FtsEX is a membrane complex widely conserved across diverse bacterial genera and involved in critical processes such as recruitment of division proteins and in spatial and temporal regulation of muralytic activity during cell division or sporulation. The component FtsX is an integral membrane protein, whereas FtsE is an ATPase and is required for the transmission of a conformational signal from the cytosol through the membrane to regulate the activity of cell wall hydrolases in the periplasm. Here, we provide the first three-dimensional (3D) structure of FtsE from the notorious pathogen S. pneumoniae, and we show that it presents all the conserved structural motifs of the NBD members of the ABC transporter family. The nucleotide-binding site is located in lobe I near the interface between the two lobes and presents the nucleotide sandwiched between the Walker A and B motifs.

FtsE was crystallized with ADP in two different crystal forms (P 1 and P 21) and with AMP-PNP, a nonhydrolyzable analog of ATP, in the space group P 21. The FtsE–AMP-PNP complex was obtained by soaking with the P 21 FtsE-ADP crystals. The ATP analog was found in two out of the three independent monomers of the P 21 crystal. Structural comparison between our ADP and AMP-PNP complexes revealed that there were no relevant structural rearrangements directly associated with AMP-PNP binding, e.g., monomer M2 in complex with ADP and that in complex with AMP-PNP were nearly identical (RMSD of 0.22 Å for 223 Cα atoms). In the presence of AMP-PNP, K43 interacts with both the β- and γ-phosphates. The γ-phosphate is further stabilized by a direct interaction with the switch histidine (H197) and with S39. The catalytic glutamate (E165) is positioned directly adjacent to the γ-phosphate, consistent with a role in ATP hydrolysis. In conclusion, the residues that recognize the ATP molecule are properly oriented, and no relevant changes were required for nucleotide exchange. Other conclusions can be drawn from our structures; in particular, we have observed that while the relaxed structure of the FtsE-ADP complex nicely fits the equivalent complex in the MacB dimer; the monomer of the FtsE–AMP-PNP complex requires rigid-body adjustment of some regions around the central β-sheet in order to get a perfect fit with the more compact structure of the MacB-ATP dimer. For instance, in our FtsE–AMP-PNP complex, the γ-phosphate is far from the Q88 residue of the Q-loop (>6 Å); however, our composite model for the same structure in the dimer indicates that Q88 would directly recognize the γ-phosphate, as also occurs in the structure of the MacB-ATP dimer.

>GSIIEMRDVVKKYDNGTTALRGVSVSVQPGEFAYIVGPSGAGKSTFIRSLYREVKIDKGSLSVAGFNLVKIKKKDVPLLRRSVGVVFQDYKLLPKKTVYENIAYAMEVIGENRRNIKRRVMEVLDLVGLKHKVRSFPNELSGGEQQRIAIARAIVNNPKVLIADEPTGNLDPDNSWEIMNLLERINLQGTTILMATHNSQIVNTLRHRVIAIENGRVVRDESKGEYGYDD[3x]5-deazatetrahydropterin | C7 H10 N4 O | 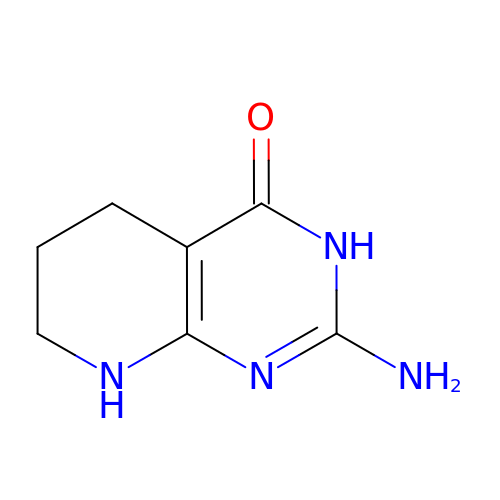PRQFDDYAWVNJMM-UHFFFAOYSA-N>PCPPTNAERLHEFHRAIGAATPERPTPPPPELLRLRQTLLDEESAEVRAEIDHLLARQAAGEALSAGDLAPLAHELADLLYVTYGALDQLGIDADAVFAEVHRANLSKASGPR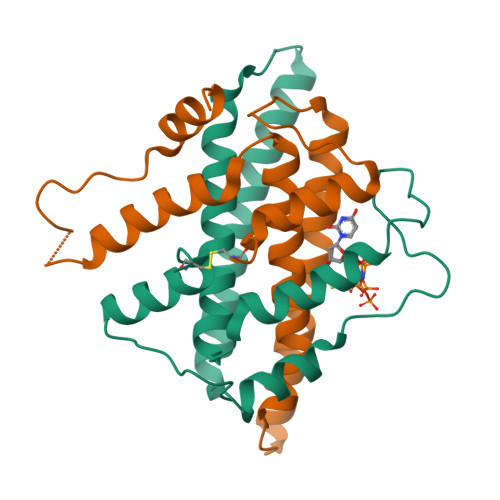RADGKQLKPEGWRPADVRGVIERLQHA[4x]In meiosis, ploidy reduction is driven by a complex series of DNA breakage and recombination events between homologous chromosomes, orchestrated by meiotic HORMA domain proteins (HORMADs). Meiotic HORMADs possess a central chromatin binding region (CBR) whose architecture varies across eukaryotic groups. Here, we determine high-resolution crystal structures of the meiotic HORMAD CBR from two diverged aquatic Holozoa, Schistosoma mansoni and Patiria miniata, which reveal tightly associated plant homeodomain (PHD) and winged helix-turn-helix (wHTH) domains. Our data reveal how meiotic HORMADs with PHD–wHTH CBRs can bind chromatin and potentially discriminate between chromatin states to drive meiotic recombination to specific chromosomal regions.

To determine these proteins’ structures and mechanisms of chromatin binding, we expressed and purified the Hop1 CBRs of two diverged aquatic Holozoa: Schistosoma mansoni (blood fluke) and P. miniata (star fish). We crystallized and determined high-resolution x-ray crystal structures of both proteins using single-wavelength anomalous diffraction (SAD) methods with the anomalous diffraction of endogenously bound Zn2+ ions. The structures show CBRs with PHD and wHTH domain tightly packed on one another in an overall configuration similar to that of the budding yeast Hop1 CBR, but lacking the HTH-C extension seen in that protein. The S. mansoni and P. miniata Hop1 CBRs are 43% identical at the amino acid level, and are nearly identical in structure, with an overall Cɑ root mean squared displacement (r.m.s.d.) of 1.4 Å over 136 residues. In contrast to the budding yeast Hop1 CBR, we find that S. mansoni and P. miniata Hop1 CBRs bind DNA via their wHTH domains through a canonical DNA binding interface. Mutation of arginine residues in each protein’s predicted DNA binding surface (R389 and R407 for S. mansoni; R463, R477, and R463 for P. miniata) to alanine resulted in a complete loss of DNA binding. We found that the P. miniata Hop1 CBR binds nucleosomes with an affinity in the low micromolar range and that alanine mutants in the PHD aromatic cage (position I residue W376) and the wHTH domain DNA binding surface (R480) each show reduced nucleosome binding. WT P. miniata Hop1 CBR bound to unmodified and H3K4me3 nucleosomes with roughly equivalent affinity, indicating the Hop1 CBR alone does not strongly discriminate between H3K4 methylation states in vitro. We also performed EMSAs with the isolated Widom 601 DNA, and observed that the wHTH domain mutant R480A, but not the PHD mutant W376A, reduced DNA binding. Overall, these data are consistent with bipartite recognition of nucleosomes by the P. miniata Hop1 CBR, with both the PHD and wHTH domain contributing to the interaction.

>[3x]MKSSHHHHHHENLYFQSNANIVRCPCGCNEDDGLMIRCEECKLWQHAVCFAIISEDDAPEQHVCNQCAKIVPRHMKPTDPYLTTLAPVVLQATCLWRRALLAATEMDRILVPNFSRRLGVEITVAHGLINRLEKEGYCQNAKGKRLGRLVNKEKLKSEGFKKYFEKK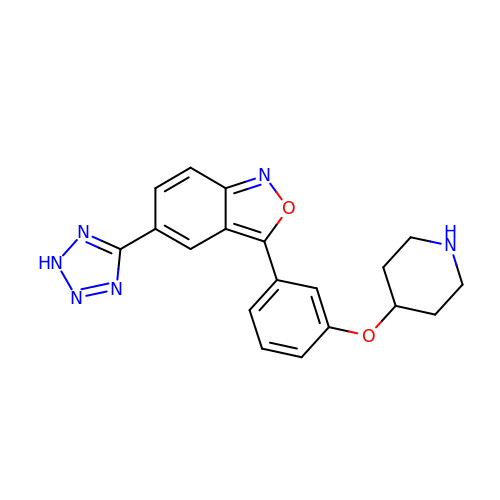(3P,5P)-3-{3-[(piperidin-4-yl)oxy]phenyl}-5-(2H-tetrazol-5-yl)-2,1-benzoxazole | C19 H18 N6 O2 | FXFKJFJHJWBHQJ-UHFFFAOYSA-N5'-[{cis-3-[2-(5-tert-butyl-1H-benzimidazol-2-yl)ethyl]cyclobutyl}(propan-2-yl)amino]-5'-deoxyadenosine | C30 H42 N8 O3 | 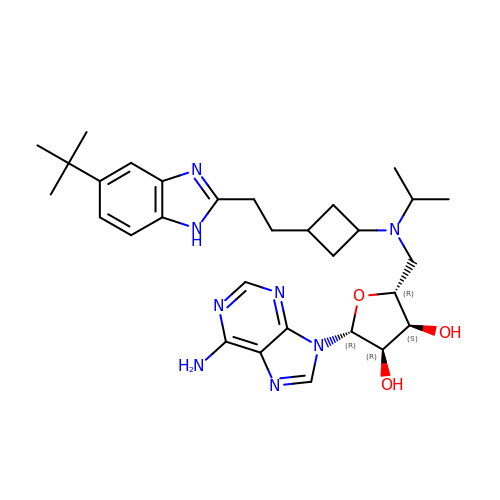LXFOLMYKSYSZQS-LURJZOHASA-N> MKLQNSFRDYTAESALFVRRALVAFLGILLLTGVLIANLYNLQIVRFTDYQTRSNENRIKLVPIAPSRGIIYDRNGIPLALNRTIYQIEMMPEKVDNVQQTLDALRSVVDLTDDDIAAFRKERARSHRFTSIPVKTNLTEVQVARFAVNQYRFPGVEVKGYKRRYYPYGSALTHVIGYVSKINDKDVERLNNDGKLANYAATHDIGKLGIERYYEDVLHGQTGYEEVEVNNRGRVIRQLKEVPPQAGHDIYLTLDLKLQQYIETLLAGSRAAVVVTDPRTGGVLALVSTPSYDPNLFVDGISSKDYSALLNDPNTPLVNRATQGVYPPASTVKPYVAVSALSAGVITRNTTLFDPGWWQLPGSEKRYRDWKKWGHGRLNVTRSLEESADTFFYQVAYDMGIDRLSEWMGKFGYGHYTGIDLAEERSGNMPTREWKQKRFKKPWYQGD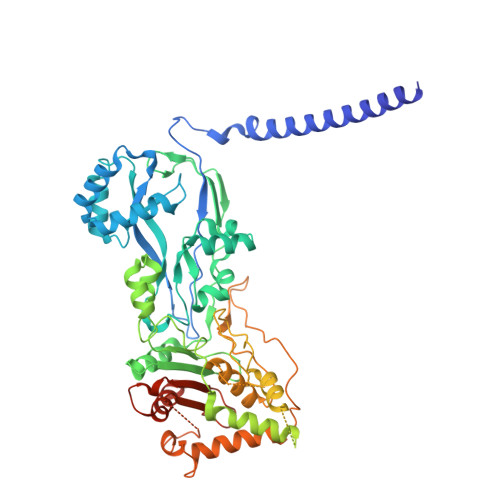TIPVGIGQGYWTATPIQMSKALMILINDGIVKVPHLLMSTAEDGKQVPWVQPHEPPVGDIHSGYWELAKDGMYGVANRPNGTAHKYFASAPYKIAAKSGTAQVFGLKANETYNAHKIAERLRDHKLMTAFAPYNNPQVAVAMILENGGAGPAVGTLMRQILDHIMLGDNNTDLPAENPAVAAAEDH>MRWQIRKLRRAEGFNVGLLIGLFIFILVGIVLLPVITSEVSSLTSGTSPAVTGTNATLLNLVPLFYILILVIVPAVLAYKMYRE[3x];> MGTKIIINVIFFDIILALLMMSFASIQPPSIANPPTVAQAQAQANITWNLTVGSINWEWLWPVFYFVDWLIWIVTTIFAVVAFIFNVFTTSLSLLASVPIVGPFLLMFAVIINFVLIWEVVKLIRGYDNPG;> MKWPLLLFTVLLIIGFTLIARAGTISLLSTPPVNPPAYSYFYIEFQFLPTNNTPQPYAIFVGPNPNNLTEVAEGYTLSNGTGYA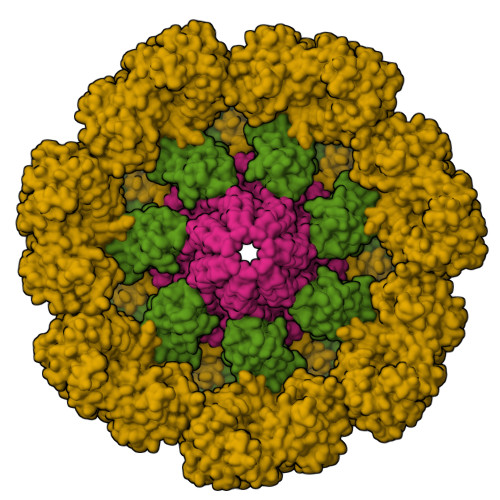RVPVINAQTEYVDIVWVNQNYTMFEIFPQIQNATTTVTLSANNNQGFSFSLPTWVSWVIGAVLMLIFMGVGWKFMGPAGLAIFGIFGLFIAMFFGLLPSYLMYVILFIVAIVGARILTKQLGGGEE;> MKRVFLLYIIGILLTLFLPLIQTQSAVSLPPLYVEDAVNAEIQQLWSKSPTGVYAFHEAPSVNNSFWPDDNAKFLESIAPWWQSYSSYVNSTLQFLQQSDVNGLFIKRFEYPLNPLQSITIGNLSGYTNGFYDIVGNPLLNSMRIATYYNPTLAVTYLFGNVVQYPNGILVNIEQGLENPITDGGFGGTGGQNPPWESLNSSSLVNDSIVSIVNNAKTYLNLTGPTFFGTPSEELQYNFPIVNVLPHYLAFQNVNGILGQYNYQGKFIPFNVTLVLQSSSINRIYLEFIWENSTSGTYVLTDIPVYFTANGQWQQVVVTVPASAWPKYWNLGALSAVPLLIGIGLDLPGSSPSQTGPTGVYVGDIATNYPTTFGPQFNVTNKGSYVVFNESWKSDSLGATFWIAYVLGQGNAIEVLASAPVNQSWIYVGYNGLATIGTGYTILETPSGILKNYQNSGNISWTYLGPNFGKWMLLSTNYAPNWIGDFQMLFIFPMAGTSNPYMDTLNNAVYMGDPTEVRNTLYFGNYTTLPGYFQWVQIAYQNDGNTSGVFGFFLIPSVDYLVNPSVIVNDMFPSSLTAYSPSSIPNYWWEAVWGENYYEGEIIYALALLGKYGNSQALQMAQQAWLSYYNQLKAYNGATYTSSLARFIMATILLYNITGNTQYSNAYTQLANWLLQYQNQSKYAYVYIPMWYHKDVDVPSVNGFATYGYIINRTAQMDVGTVISGTSIGLNFFEDIPLNTSYGIYLLTNGTGKLPFTYQNVLNVSGTFITYLYMNGGGTATTANITITVQIAYNGNVLQTIGTAAVDNVPIQPGGISGSPPFYPVKIVVPVLTTVNAPPGSTLIIGWNIKAPQTVYVLIDSTNGPSNVTIPLSWPNPFYGLFTIPKIYNPNPGVHNYPQPYFLDISAMAGQAMMALYAVTKNITYLLDAQLVMNAIHYGPVPMPTYGILGVPNPPVEPRLWVYANYSTVDADYYTYKSELVSEFGDAIGNNTLASLAISRVWQRTSYTYPTSYIYYVARYGSGLQMNSETQPWGDVATQFYVNTWSPSNLDLFWASLPNNNYITNQTWNGTALFIHLYAYQQSQVQLIFLTTTVNFNVLVNGNYTNYEANHQIMQIAPTLEPGPNTIIIIPNPKNQVSQNTNISTTTTTSPLSNAISGLGITLTQNELMLLGFVIYFVIIMVTYGVSRNKTITVLSSIVAVAIVYALALWPTYMAFILGAVGFFMLFYSISRREEE The highly conserved coiled-coil domain-containing protein 61 (CCDC61, also known as variable flagellar number 3, VFL3) is one of these understudied proteins. Here, we identify CCDC61 as a highly conserved paralog of SAS6, a key organizer of the central scaffold around which centrioles are formed (Leidel et al., 2005). Our crystal structures of CCDC61 demonstrate that it adopts a SAS6-like fold and forms oligomers through two homodimerization domains in a similar way to SAS6: an N-terminal globular head and a parallel coiled-coil domain. Further analysis of CCDC61 reveals that its coiled-coil domains are capable of directly interacting with microtubules.

To find out whether CCDC61 can form a ring in a similar manner to SAS6, we determined the crystal structure of zebrafish CCDC61 (residues 1–170; zCCDC611−170), which contains both its head and parts of its coiled-coil domain, by X-ray crystallography at a resolution of 2.9 Å. In the crystal, zCCDC611−170 formed a homo-tetramer mediated by the head-to-head and the coiled-coil dimer interactions in an arrangement that would not be compatible with the assembly of a ring. A filament model of zCCDC611−170 suggests that CCDC61 would be able to form protofilaments with a left-handed 3-fold screw axis along the filament, the helical rise of which is ∼80 Å. However, instead of the spiral/ring assemblies observed with SAS6, CCDC61 assembles into linear filaments with 3-fold, left-handed screw axes in vitro. To further confirm higher-order oligomer formation of zCCDC611−170 in solution, we subjected this construct, as well as its F129E/D130A mutant that disrupts the head-to-head interaction in zCCDC61, to size-exclusion chromatography with multi-angle light scattering analysis. In this experiment, the His6-lipoyl domain tag of each construct was retained to stabilize the corresponding proteins at high concentrations. The results shown in Figure 2D demonstrate that the wild-type, but not the head-to-head dimerization-deficient mutant, was able to form higher-order oligomers beyond the coiled-coil-mediated dimer. Comparison of the structures of zCCDC61, SAS6 (Leishmania major [lmSAS6]), and Caenorhabditis elegans (ceSAS6) and human XRCC4/XLF by superposition of their head domains showed that the difference between the exact higher-order assemblies formed by these proteins originates from (1) altered relative orientation angles between their head domains and (2) altered relative orientation angles between the head and coiled-coil domains. Intriguingly, in the filaments formed by CCDC61 in vitro, the distance between the projecting coiled-coil domains of CCDC61 that point in the same direction is about 24 nm, which corresponds to three times the 8-nm repeat of tubulin dimers in microtubules. This periodicity might facilitate microtubule interaction by the CCDC61 coiled-coil domain.

>GGSMEVGTVVQEEMKFRGSEFAVKVEMAERLLIVEISDVVTADQWRGEFGPAYIEDLTRKTGNFKQFPVFCSMLESAVHKSSDSVTLDLLTYSDLELLRNRKAGVVGRPRAQPQSPALSAKRYLILIYTVEFDRIHYPLPLPYLGKPDPAELQKEIRALRSELKTLGLRGDHK[2x]>[4x]MHHHHHHENLYFQGRNVALITGITGQDGSYLAEFLLEKGYEVHGIVRRSSSFNTGRIEHLYKNPQAHIEGNMKLHYGDLTDSTCLVKIINEVKPTEIYNLGAQSHVKISFDLAEYTADVDGVGTLRLLDAVKTCGLINSVKFYQASTSELYGKVQEIPQKETTPFYPRSPYGAAKLYAYWIVVNFREAYNLFAVNGILFNHESPRRGANFVTRKISRSVAKIYLGQL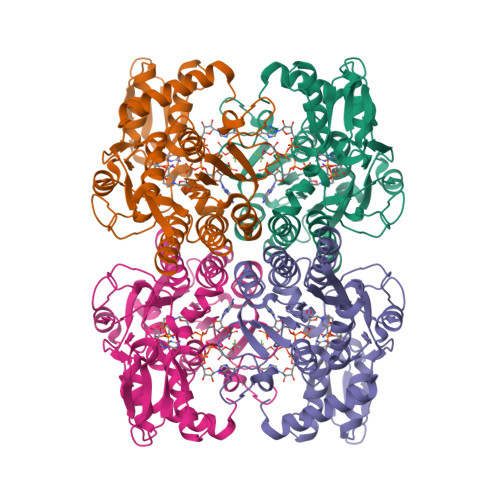ECFSLGNLDAKRDWGHAKDYVEAMWLMLQNDEPEDFVIATGEVHSVREFVEKSFLHIGKTIVWEGKNENEVGRCKETGKVHVTVDLKYYRPTEVDFLQGDCTKAKQKLNWKPRVAFDELVREMVHADVELMRTNPNA>[2x]APRKFFVGGNWKMNGDKKSLGELIHTLNGAKLSADTEVVCGAPSIYLDFARQKLDAKIGVAAQNCYKVPKGAFTGEISPAMIKDIGAAWVILGHSERRHVFGESDELIGQKVAH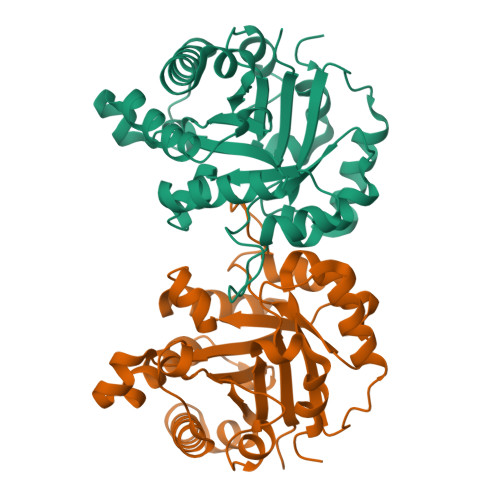ALAEGLGVIACIGEKLDEREAGITEKVVFEQTKAIADNVKDWSKVVLAYEPVWAIGTGLWATPQQAQEVHEKLRGWLKSHVSDAVAQSTRIIYGGSVTGGNCKELASQHDVDGFLVGGASLKPEFVDIINAKH> MGSS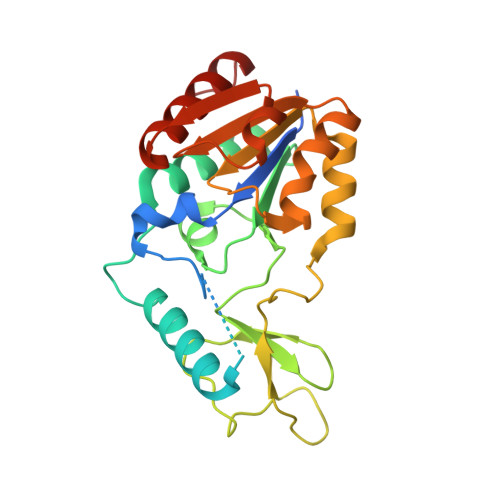HHHHHHSQDPKPRVLVLTGAGISAESGIRTFRAADGLWEEHRVEDVGTPEGFDRDPELVQAFANARRRQLQQPEIQPNAAHLALAKLQDALGDRFLLVTQNLDNLHERAGNTNVIHMHGELLKVRCSQSGQVLDWTGDVTPEDKCHCCQFPAPLRPHYVWFGEMPLGMDEIYMALSMADIFIAIGTSGHVYPAAGFVHEAKLHGAHTVELNLEPSQVGNEFAEKYYGPASQVVPEFVEKLLKGLKAGSIA> MRGSHHHHHHGSAVSAKIEIYTWSTCPFCMRALALLKRKGVEFQEYCIDGDNEAREAMAARANGKRSLPQIFIDDQHIGGCDDIYALDGSGKLDPLLHS

In the case of the glutaredoxin that is the focus of this study, glutaredoxin A from the cyanobacterium Synechocystis sp. PCC 6803 serves as the preferred electron donor for the 2-electron reduction of arsenate to arsenite, catalyzed by arsenate reductase. As part of the thioredoxin superfamily, glutaredoxin A shares the characteristic thioredoxin fold. The structure of the wild-type protein is comprised of the major protein secondary structure elements: four α-helical segments, and four mixed parallel: anti-parallel β-strands that form a single β-pleated sheet. Our random mutagenesis approach has yielded four new crystal structures of glutaredoxin A, one for each of the following variants: R27L, A75I, A79S, and P84R.

Due to the location of Ala75, one might have predicted that changes in structure and function observed for the A75I and the A79S variants would be subtle. These replacements are located at the extreme C-terminus of the protein in α-helix 4, and both are exposed to the outside surface of the helix. Neither is involved in crystal packing interactions nor core packing interactions, and therefore, these positions are predicted to be highly tolerant of modification. However, in the case of the A79S mutant, there are minor structural changes observed in the geometry of α-helix 4. There is a measurable decrease in the twist of the helix, a decrease in the helix-bending angle of α-helix 4. The significance of these minor changes remains to be explored. The R27L crystal structure lacks two neighbors; the A75I and A79S mutant have no net differences, while the P84R mutant adds three possible interactions.6-[4-[(5~{S})-5-[3,5-bis(fluoranyl)phenyl]pyrazolidin-1-yl]carbonylpiperidin-1-yl]pyrimidine-4-carbonitrile | C20 H20 F2 N6 O | 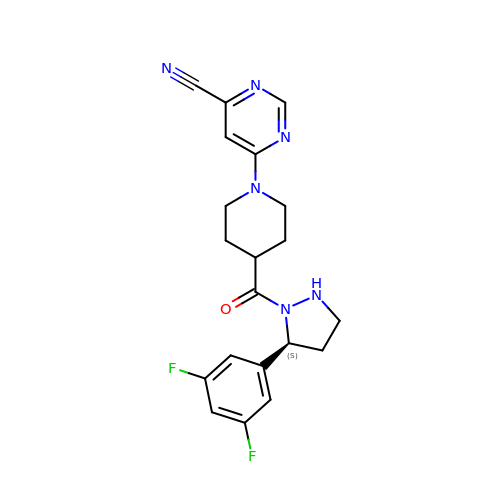PZXPEVAQKNYNRX-SFHVURJKSA-N>APQQINDIVHRTITPLIEQQKIPGMAVAVIYQGKPYYFTWGYADIAKKQPVTQQTLFELGSVSRTFTGVLGGDAIARGEIKLSDPTTKYW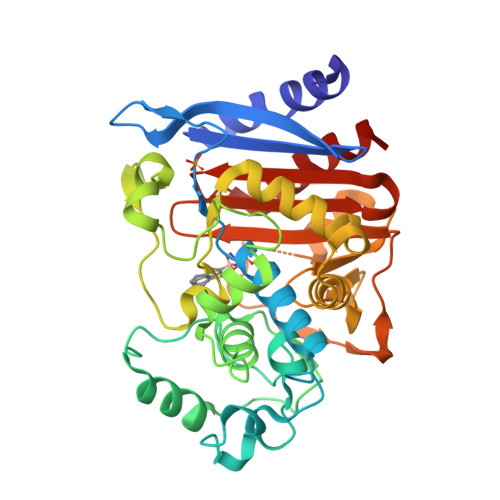PELTAKQWNGITLLHLATYTAGGLPLQVPDEVKSSSDLLRFYQNWQPAWAPGTQRLYANSSIGLFGALAVKPSGLSFEQAMQTRVFQPLKLNHTWINVPPAEEKNYAWGYREGKAVHVSPGALDAEAYGVKSTIEDMARWVQSNLKPLDINEKTLQQGIQLAQSRYWQTGDMYQGLGWEMLDWPVNPDSIINGSDNKIALAARPVKAITPPTPAVRASWVHKTGATGGFGSYVAFIPEKELGIVMLANKNYPNPARVDAAWQILNALQ[2x]>[2x]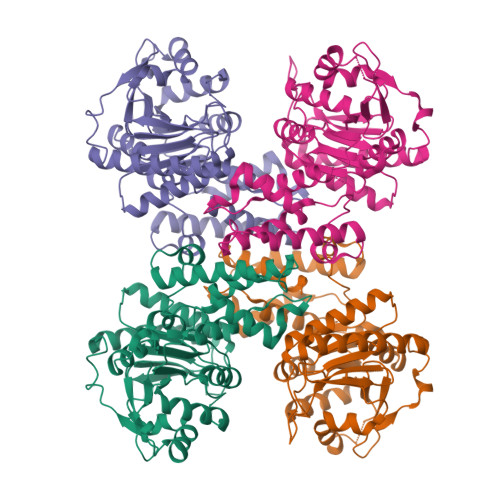DSLIMFLVEIFRSLFVSNCIDKNIDNVLLSIEEMFIDHYYNPQHSRLKYLIDDVGIFFTKLPITKAFHTYNKKYRITKRLYAPPTFNEVRHILNLAQILSLEEGLDLLTFDADETLYPDGHDFNDEVLASYISCLLKKMNIAIVTAASYNNDAEKYQKRLENLLKYFSKHNIKDGSYKNFYVMGGESNYLFKCNEEATLYSVPENEWRHYKKFVDYDTVQEILNISEKCLEKVIKDFGLCAQIQRKEKSIGLVPNKIPSLNIKNEQKNYMIKYEVLEEAVIRIKKEIIKNKITAPYCAFNGGQDLWVDVGNKAEGLLILQKLLKIQKKKCCHIGDQFLHSGNDFPTRFCSLTLWVSNPQETKACLKSIMHLNIKSFIPEVLYENQ> GSHMLTNLVAEPFAKLEQDFGGSIGVYAMDTGSGATVSYRAEERFPLCSSFKGFLAAAVLARSQQQAGLLDTPIRYGKNALVPWSPISEKYLTTGMTVAELSAAAVQYSDNAAANLLLKELGGPAGLTAFMRS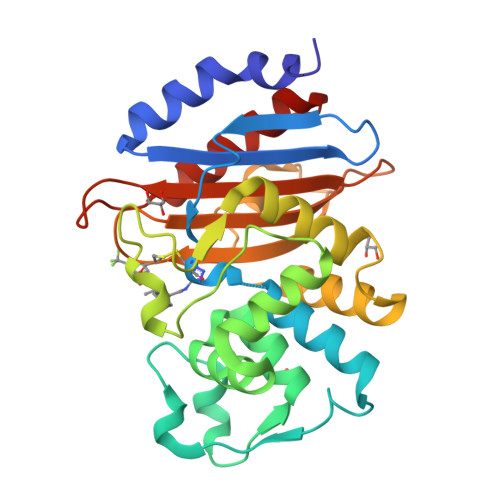IGDTTFRLDRWELELNSAIPGDARDTSSPRAVTESLQKLTLGSALAAPQRQQFVDWLKGNTTGNHRIRAAVPADWAVGDKTGTCGVYGTANDYAVVWPTGRAPIVLAVYTRAPNKDDKHSEAVIAAAARLALEGLGVNG6-{[4-(4-methylpiperazin-1-yl)phenyl]amino}-2-(prop-2-en-1-yl)-1-{6-[(1S)-2,2,2-trifluoro-1-hydroxyethyl]pyridin-2-yl}-1,2-dihydro-3H-pyrazolo[3,4-d]pyrimidin-3-one 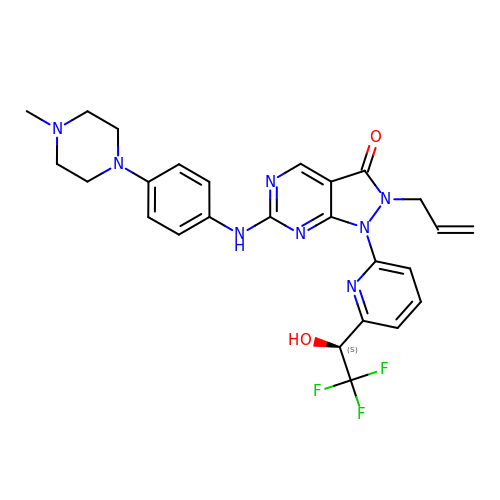| C26 H27 F3 N8 O2 | DQUHCAHRQQRKGR-QFIPXVFZSA-N>MLSRKGIIPEEYVLTRLAEDPTEPRYRTRERRARFVSKKGNCNVAHKNIREQGRFLQDVFTTLVDLKWPHTLLIFTMSFLCSWLLFAMVWWLIAFAHGDLAPGEGTNVPCVTSIHSFSSAFLFSIEVQVTIGFGGRMVTEECPLAILILIVQNIVGLMINAIMLGCIFMKTAQAHRRAETLIFSKHAVITPRHGRLCFMLRVGDLRKSMIISATIHMQVVRKTTSPEGEVVPLHQVDIPMENGVGGNSIFLVAPLIIYHVIDSNSPLYDLAPSDLHHHQDLEIIVILEGVVETTGITTQARTSYLADEILWGQRFVPIVAEEDGRYSVDYSKFGNTVKVPTPLCTARQLDEDRSLLDALTLASSRGPLRKRSVAVAKAKPKFSISPDSLS[4x];>MPLAFCGTENHSAAYRVDQGVLNNGCFVDALNVVPHVFLLFITFPILFIGWGSQSSKVHIHHSTWLHFPGHNLRWILTFILLFVLVCEIAEGILSDGVTESRHLHLYMPAGMAFMAAITSVVYYHNIETSNFPKLLIALLIYWTLAFITKTIKFVKFYDHAIGFSQLRFCLTGLLVILYGMLLLVEVNVIRVRRYIFFKTPREVKPPEDLQDLGVRFLQPFVNLLSKGTYWWMNAFIKTAHKKPIDLRAIAKLPIAMRALTNYQRLCVAFDAQARKDTQSPQGARAIWRALCHAFGRRLILSSTFRILADLLGFAGPLCIFGIVDHLGKENHVFQPKTQFLGVYFVSSQEFLGNAYVLAVLLFLALLLQRTFLQASYYVAIETGINLRGAIQTKIYNKIMHMSTSNLSMGEMTAGQICNLVAIDTNQLMWFFFLCPNLWTMPVQIIVGVILLYYILGVSALIGAAVIILLAPVQYFVATKLSQAQRTTLEHSNERLKQTNEMLRGMKLLKLYAWESIFCSRVEVTRRKEMTSLRAFAVYTSISIFMNTAIPIAAVLITFVGHVSFFKESDLSPSVAFASLSLFHILVTPLFLLSSVVRSTVKALVSVQKLSEFLSSAEIREEQCAPREPAPQGQAGKYQAVPLKVVNRKRPAREEVRDLLGPLQRLAPSMDGDADNFCVQIIGGFFTWTPDGIPTLSNITIRIPRGQLTMIVGQVGCGKSSLLLATLGEMQKVSGAVFWNSNLPDSEGEDPSSPERETAAGSDIRSRGPVAYASQKPWLLNATVEENITFESPFNKQRYKMVIEACSLQPDIDILPHGDQTQIGERGINLSGGQRQRISVARALYQQTNVVFLDDPFSALDVHLSDHLMQAGILELLRDDKRTVVLVTHKLQYLPHADWIIAMKDGTIQREGTLKDFQRSECQLFEHWKTLMNRQDQELEKETVMERKASEPSQGLPRAMSSRDGLLLDEEEEEEEAAESEEDDNLSSVLHQRAKIPWRACTKYLSSAGILLLSLLVFSQLLKHMVLVAIDYWLAKWTDSALVLSPAARNCSLSQECDLDQSVYAMVFTLLCSLGIVLCLVTSVTVEWTGLKVAKRLHRSLLNRIILAPMRFFETTPLGSILNRFSSDCNTIDQHIPSTLECLSRSTLLCVSALTVISYVTPVFLVALLPLAVVCYFIQKYFRVASRDLQQLDDTTQLPLVSHFAETVEGLTTIRAFRYEARFQQKLLEYTDSNNIASLFLTAANRWLEVCMEYIGACVVLIAAATSISNSLHRELSAGLVGLGLTYALMVSNYLNWMVRNLADMEIQLGAVKRIHALLKTEAESYEGLLAPSLIPKNWPDQGKIQIQNLSVRYDSSLKPVLKHVNTLISPGQKIGICGRTGSGKSSFSLAFFRMVDMFEGRIIIDGIDIAKLPLHTLRSRLSIILQDPVLFSGTIRFNLDPEKKCSDSTLWEALEIAQLKLVVKALPGGLDAIITEGGENFSQGQRQLFCLARAFVRKTSIFIMDEATASIDMATENILQKVVMTAFADRTVVTIAHRVHTILSADLVMVLKRGAILEFDKPETLLSQKDSVFASFVRADK[4x]

ATP-sensitive potassium (KATP) channels are unique hetero-octameric complexes each composed of four inwardly rectifying Kir6 channel subunits and four sulfonylurea receptor (SUR) subunits belonging to the ATP binding cassette (ABC) transporter protein family. In pancreatic β-cells, KATP channels formed by Kir6.2 and SUR1 are gated by intracellular ATP and ADP, with ATP inhibiting channel activity while Mg2+-complexed ATP and ADP stimulating channel activity. During glucose stimulation, the intracellular ATP to ADP ratio increases following glucose metabolism, which favors channel closure by ATP, resulting in membrane depolarization, Ca2+ influx, and exocytosis of insulin granules. All sulfonylureas stimulate insulin secretion to reduce plasma glucose levels by inhibiting the activity of β-cell KATP channels.

To obtain a structure of KATP channels bound to GBC and ATP, channels comprising a rat Kir6.2 and FLAG-tagged hamster SUR1 (96% and 95% sequence identity to human sequences, respectively) were expressed in rat insulinoma INS-1 832/13 cells, affinity purified, and imaged in the presence of 1 mM ATP (no Mg2+) and 1 µM GBC. Particles from this class were further classified and refined using Frealign, which yielded a map with improved resolution of 3.63 Å. In our new structure, constrictions in the selectivity filter (T130), bundle crossing (F168), and the G-loop (G295, I296) are clearly seen to indicate a closed pore. SUR1 is found in an ‘inward-facing’ conformation, with NBDs clearly separated and the vestibule formed by TMD1/TMD2 open towards the cytoplasm. We have previously reported the location of the ATP-binding site at the interface of the cytoplasmic N- and C-terminal domains from two adjacent subunits, giving four equivalent sites for the Kir6.2 tetramer. The pocket itself is formed by the overlap of three distinct cytoplasmic structures: an N-terminal peptide (binding residues N48 and R50; subunit A) immediately before the Kir channel ‘slide helix’; a C-terminal β-sheet (I182 and K185; subunit B) immediately following the TMD-CTD tether helix; and a short, solvent-exposed helical segment (Y330, F333, G334; subunit B). The α- phosphate of ATP is coordinated by the main-chain nitrogen of G334 and K185, while the β- and γ-phosphates are coordinated by side-chain nitrogens of K185 and R50, respectively. In the current reconstruction we find well defined, non-protein density within the TMDs of SUR1, with a size and shape which closely matches that of a GBC molecule. A primary anchor is composed of two arginine residues, R1246 and R1300, which coordinate each oxygen of the sulfonyl group. Each nitrogen of the urea moiety is coordinated by T1242 and N1245, and the adjacent benzene and cyclohexyl groups (adjacent to the sulfonyl and urea groups, respectively) are stabilized by a series of hydrophobic interactions contributed by TM helices from both TMD1 (TM6, 7, 8) and TMD2 (TM16).>GPVSVANHLGEDAGHLALRRDVYSGLQKTPKSLPPKWFYDTV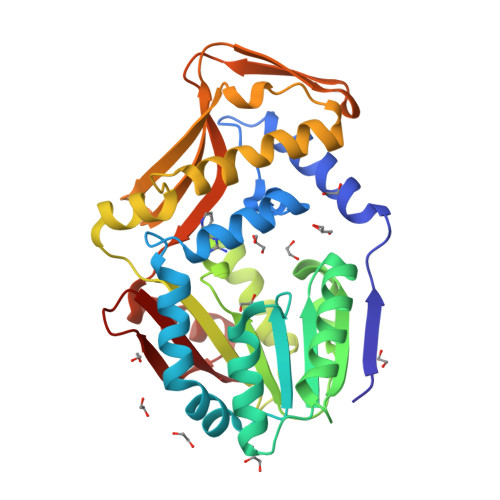GSELFDQITRLPEYYPTRAEAEILRARSAEVASACRADTLVELGSGTSEKTRMLLDALRHRGSLRRFVPFDVDASVLSATATAIQREYSGVEINAVCGDFEEHLTEIPRGGRRLFVFLGSTIGNLTPGPRAQFLTALAGVMRPGDSLLLGTDLVKDAARLVRAYDDPGGVTAQFNRNVLAVINRELEADFDVDAFQHVARWNSAEERIEMWLRADGRQRVRVGALDLTVDFDAGEEMLTEVSCKFRPQAVGAELAAAGLHRIRWWTDEAGDFGLSLAAK[2x]>MNSLTLTSDQENALEGMKAFCANSLDKNWPAALLQGYAGTGKTTLLGVLVSSLVEKGYKVAVTAPTNKAVSVLMEKVPDASCHATIHSLLGLALQEEGETQKLVSSGTSCVNDFDVVIVDECSMIGADLLSMIRGRPKFIFVGDPAQLPPVNEIFSPVFRSVGLRWSLSKIVRQAEGNAIIDLSAEIRLKSEEGVPMTLEDIKSILEGKLEACCMSGIDLVSALTHEWKEGRDSRILAWRNATVDFYNRAIFSSLYPDATTPFVPGQTAIVGSSFEVDPDAHVRLDTSEEVTILSLEPGERLGVPVFLAR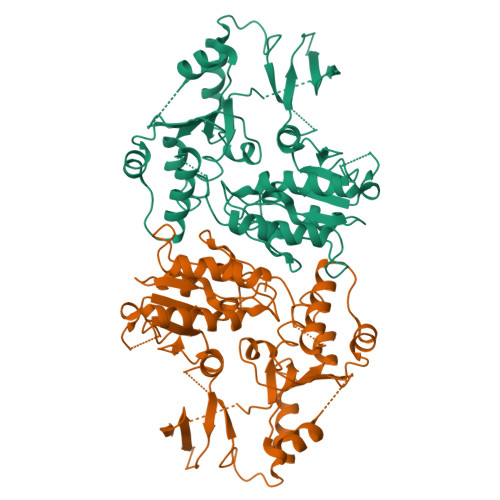VQRASGETWTLPIPRSSSDFAREVKASFSEWRFWKNQVKASPSASEASEADRKASAFLKKGWALKKGIADLRHPWAMTVHKAQGSTYDTVFVDWNDLRAIPSDDFLRILYTAVTRPSRYLAICH[2x]2-[2-methyl-1-(naphthalen-1-ylmethyl)-3-oxamoyl-indol-4-yl]oxyethanoic acid | C24 H20 N2 O5 | 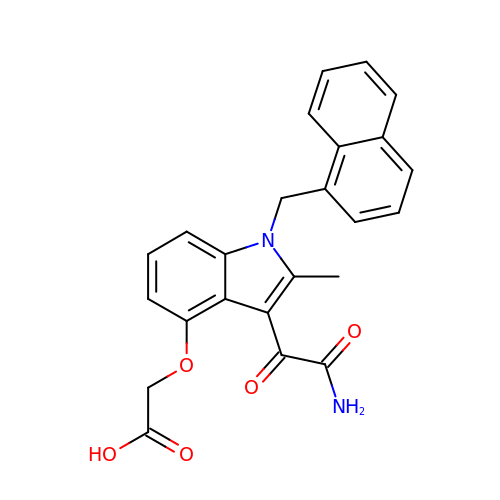OCZWKLXXLNWSDH-UHFFFAOYSA-N> MTITLDICEKDIIVSTEIDDIIFTSSPLDITYDEQERIKHKLILESFRYHYNNNEDYKSFCNTQGVDENISSLDDIPVFPTSMFKYAKICTADESNIENWFTSSGTSGVKSHIARDRVSIERLLGSVNYGMKYLGSFHENQLELVNMGPDRFNAKNVWFKYVMSLVELLYPTTFTVNNDEIDFELTIKSLKEIYNKGKGICLIGPPYFIYLLCQYMKENDIEFNAGNRIFII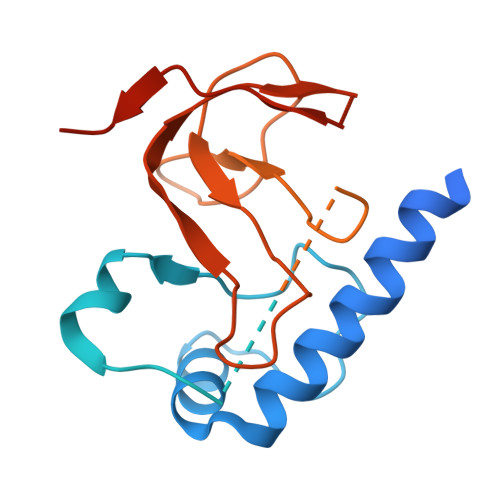TGGGWKTKQKQALNRQDFNQLLMETFHLAHESQIRDTFNQVELNTCFFEDNRQRKHVPPWVYARALDPVTLKPVEDGQEGLISYMDASSTSYPTFIVTDDIGIIHTIKAPDPHQGTTIDIVRRLNTREQKGCSLSMSSGLK>YFQSMGGSYKVILYELE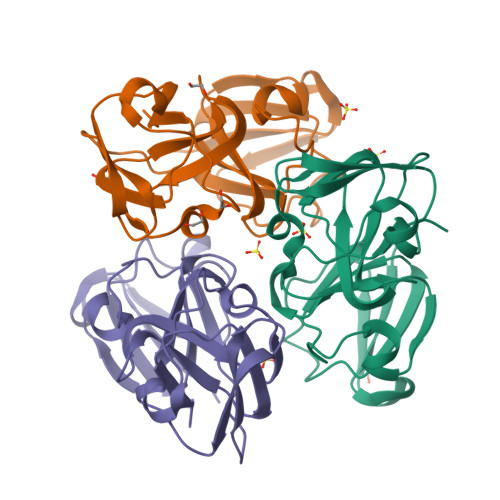NFQGKRCELSAECPSLTDSLLEKVGSIQVESGPWLAFESRAFRGEQFVLEKGDYPRWDAWSNSRDSDSLLSLRPLNIDSPHHKLHLFENPAFSGRKMEIVDDDVPSLWAHGFQDRVASVRAINGTWVGYEFPGYRGRQYVFERGEYRHWNEWDASQPQLQSVRRIRD[3x]> MKKIANYLLIEKTDDRYTISMTPELQDDIGTIGYAEFTDNDHLAVDDIILNLEASKTVMSVLSPLAGAVVERNEAATLTPTLLNSEKAEENWIVVLTDVDQAAFDALEDAGSGHHHHHHH

In this study, we report on the identification of a distinct class of sirtuins (SirTMs) found primarily in pathogenic microorganisms and show that these function as protein ADP-ribosyl transferases. Members of this sirtuin class are genetically linked to a specific subclass of macrodomain proteins, which reverse the sirtuin catalyzed ADP-ribosylation. Moreover, we show that in Staphylococcus aureus and Streptococcus pyogenes the sirtuin-mediated ADP-ribosylation is dependent on another posttranslational modification—lipoylation.

To better understand the spatial relationship between ADP-ribosylation and lipoylation attachment sites, we determined the crystal structure of SpyGcvH-L. The structure contains residues 1–110 and is comprised of a barrel-sandwich hybrid formed by two β sheets flanked by short α helices. In comparison with previously solved H-proteins (RMSDs for all Cα atoms ranging from 0.575–1.14 Å), the most striking differences observed in SpyGcvH-L are (1) the position of the β4/β5 loop (residues 38–40), which diverges from the consensus path by ∼6 Å as a consequence of the presence of Arg72 in the β8 strand (a position usually occupied by Val or Ile); and (2) the absence of a C-terminal α helix. Intriguingly, the missing α helix, which is held in place by electrostatic contacts between four conserved residues in the canonical GcvHs, would occlude residues implicated in ADP-ribose attachment in SpyGcvH-L (Glu24 and Asp27). The absence of the steric hindrance imposed by this α helix may be a prerequisite for the GcvH-L/SirTM interaction and thus could account for the high substrate specificity of SirTMs. Mutagenesis showed that the lipoyl-attachment site is Lys56 within the conserved Ex(2)Kx(10)G motif (Fujiwara et al., 1991; Spalding and Prigge, 2009). Only extended exposure revealed slight ADP-ribosylation of E24A, whereas no ADPr incorporation could be detected for D27A. These findings suggest that Asp27 is the likely ADPr attachment side, but further indicates involvement of Glu24 in the ADP-ribosylation mechanism. On the other hand, Glu24 is only present in GcvH-L homologs. Since ADP-ribosylation is a known modification influencing protein function and interactions (Barkauskaite et al., 2013), it is interesting to speculate that the MARylation state of GcvH-L might regulate the availability of the lipoyl moiety for redox reactions. This idea is supported by our finding that the ADPr attachment site is in close structural proximity to the lipoylation site. Strikingly, SirTMs show absolute selectivity for the lipoylated GcvH-L. Altogether, these data show that lipoylated, full-length GcvH-L is required as substrate in the ADP-ribosylation reaction.>MTSNLIKFDDQNKVFHLHNKQISYLLSIEDGGTLSHLYFGGAVKNYNNQLKYPRLDRGFSGNLPESLDRTFSRDSLPKEYSSAGEMDFHTPATIVRNPDGSNALFLAYKSYKIEDGKPDLKGLPHSWTKEDDEAQTLIVTLEDKVSKLEYDLLYTIYRDRPVIVRSVQVHNHGEEAVYLEKVASMQMDYVDKDFEVITLPGAHANERRVQRENIGQGIKVFSSYRGTSSHQMNPFMALVDHDTNEFMGEAYGFALAYSGNHKFEVERDQFGQIHVNTGINDYNFKWKLNPNEEFQTPEVLMVYSDQGLNKMSQAFHSLIHERIMRSKFKDQIRPVLVNNWEATYFDFNEDKLKTIVDKAKKLGLEMFVLDDGWFGHRDDDNSSLGDWKVYKKKFPNGLGHFADYVHEQGLKFGLWFEPEMISY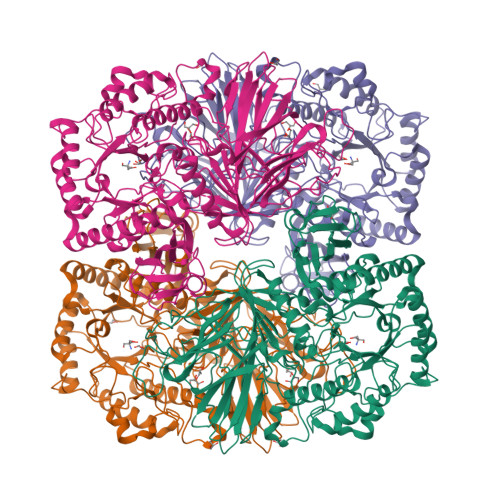ESNLYKEHPDYLMHVPGRKPCPSRNQYVLELGRKEVRDNIFEQMVKILDSKKIDYIKWDMNRSLSDIYESDLPADQQGEAYHRYVLGYYDLLNKLVTRYPDILFEGCSGGGGRFDVGQAYYTPQIWASDNTDAIERLKIQYGTSLVYPQSMMTSHVSVSPNEQNGRITPFNTRGAVAMWGDLGYELDLTKMSDEESDQVVKQVTEYKKIREVTQFGTLYRLKASASNQCAWMMVDSNKNEAVVTVVNVMAHAQPYCTKTKLAGLDPDKRYKNLETDEVFGGDELMHLGFYDPIERGDFKAKMYHFKAIN[4x]>MRGSHHHHHHGSWETEERPRTREEESHFYAGGQVYPGEASRVSVADHSLHLSKAKISKPAPYWEGTAVIDGEFKELKLTDYRGKYLVFFFYPLDFTFVSPTEIIAFGDRLEEFRSINTEVVACSVDSQFEHLAW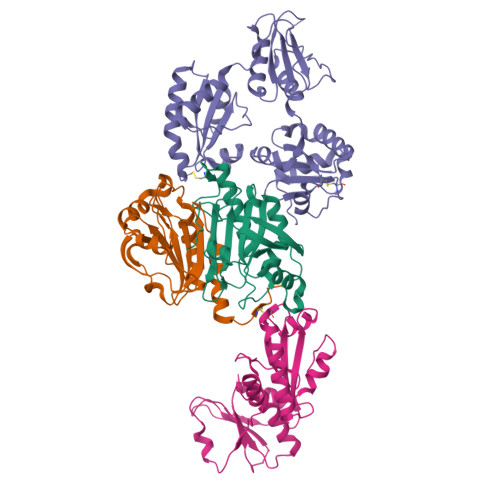INTPRRQGGLGPIRIPLLSDLTHQISKDYGVYLEDSGHTLRGLFIIDDKGILRQITLNDLPVGRSVDETLRLVQAFQYTDKHGEVCPAGWKPGSETIIPDPAGKLKYFDKLN[2x];>[2x]GPLGSEITSLDTENIDEILNNADVALVNFYADWCRFSQMLHPIFEEASDVIKEEFPNENQVVFARVDCDQHSDIAQRYRISKYPTLKLFRNGMMMKREYRGQRSVKALADYIRQQKSDPIQEIRDLAEITTLDRSKRNIIGYFEQKDSDNYRVFERVANILHDDCAFLSAFGDVSKPERYSGDNIIYKPPGHSAPDMVYLGAMTNFDVTYNWIQDKCVPLVREITFENGEELTEEGLPFLILFHMKEDTESLEIFQNEVARQLISEKGTINFLHADCDKFRHPLLHIQKTPADCPVIAIDSFRHMYVFGDFKDVLIPGKLKQFVFDLHSGKLHREFHHGPDPTDTAPGEQAQDVASSPPESSFQKLAPSEYRYTLLRDRDEL>[4x]MLSRKGIIPEEYVLTRLAEDPTEPRYRTRERRARFVSKKGNCNVAHKNIREQGRFLQDVFTTLVDLKWPHTLLIFTMSFLCSWLLFAMVWWLIAFAHGDLAPGEGTNVPCVTSIHSFSSAFLFSIEVQVTIGFGGRMVTEECPLAILILIVQNIVGLMINAIMLGCIFMKTAQAHRRAETLIFSKHAVITLRHGRLCFMLRVGDLRKSMIISATIHMQVVRKTTSPEGEVVPLHQVDIPMENGVGGNSIFLVAPLIIYHVIDSNSPLYDLAPSDLHHHQDLEIIVILEGVVETTGITTQARTSYLADEILWGQRFVPIVAEEDGRYSVDYSKFGNTVKVPTPLCTARQLDEDRSLLDALTLASSRGPLRKRSVAVAKAKPKFSISPDSLS;> MPLAFCGTENHSAAYRVDQGVLNNGCFVDALNVVPHVFLLFITFPILFIGWGSQSSKVHIHHSTWLHFPGHNLRWILTFILLFVLVCEIAEGILSDGVTESRHLHLYMPAGMAFMAAITSVVYYHNIETSNFPKLLIALLIYWTLAFITKTIKFVKFYDHAIGFSQLRFCLTGLLVILYGMLLLVEVNVIRVRRYIFFKTPREVKPPEDLQDLGVRFLQPFVNLLSKGTYWWMNAFIKTAHKKPIDLRAIAKLPIAMRALTNYQRLCVAFDAQARKDTQSPQGARAIWRALCHAFGRRLILSSTFRILADLLGFAGPLCIFGIVDHLGKENHVFQPKTQFLGVYFVSSQEFLGNAYVLAVLLFLALLLQRTFLQASYYVAIETGINLRGAIQTKIYNKIMHMSTSNLSMGEMTAGQICNLVAIDTNQLMWFFFLCPNLWTMPVQIIVGVILLYYILGVSALIGAAVIILLAPVQYFVATKLSQAQRTTLEHSNERLKQTNEMLRGMKLLKLYAWESIFCSRVEVTRRKEMTSLRAFAVYTSISIFMNTAIPIAAVLITFVGHVSFFKESDLSPSVAFASLSLFHILVTPLFLLSSVVRSTVKALVSV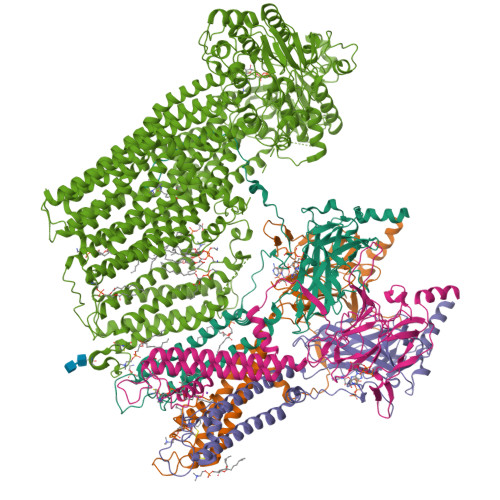QKLSEFLSSAEIREEQCAPREPAPQGQAGKYQAVPLKVVNRKRPAREEVRDLLGPLQRLAPSMDGDADNFCVQIIGGFFTWTPDGIPTLSNITIRIPRGQLTMIVGQVGCGKSSLLLATLGEMQKVSGAVFWNSNLPDSEGEDPSSPERETAAGSDIRSRGPVAYASQKPWLLNATVEENITFESPFNKQRYKMVIEACSLQPDIDILPHGDQTQIGERGINLSGGQRQRISVARALYQQTNVVFLDDPFSALDVHLSDHLMQAGILELLRDDKRTVVLVTHKLQYLPHADWIIAMKDGTIQREGTLKDFQRSECQLFEHWKTLMNRQDQELEKETVMERKASEPSQGLPRAMSSRDGLLLDEEEEEEEAAESEEDDNLSSVLHQRAKIPWRACTKYLSSAGILLLSLLVFSQLLKHMVLVAIDYWLAKWTDSALVLSPAARNCSLSQECDLDQSVYAMVFTLLCSLGIVLCLVTSVTVEWTGLKVAKRLHRSLLNRIILAPMRFFETTPLGSILNRFSSDCNTIDQHIPSTLECLSRSTLLCVSALTVISYVTPVFLVALLPLAVVCYFIQKYFRVASRDLQQLDDTTQLPLVSHFAETVEGLTTIRAFRYEARFQQKLLEYTDSNNIASLFLTAANRWLEVCMEYIGACVVLIAAATSISNSLHRELSAGLVGLGLTYALMVSNYLNWMVRNLADMEIQLGAVKRIHALLKTEAESYEGLLAPSLIPKNWPDQGKIQIQNLSVRYDSSLKPVLKHVNTLISPGQKIGICGRTGSGKSSFSLAFFRMVDMFEGRIIIDGIDIAKLPLHTLRSRLSIILQDPVLFSGTIRFNLDPEKKCSDSTLWEALEIAQLKLVVKALPGGLDAIITEGGENFSQGQRQLFCLARAFVRKTSIFIMDEATASIDMATENILQKVVMTAFADRTVVTIAHRVHTILSADLVMVLKRGAILEFDKPETLLSQKDSVFASFVRADK> MKFKLNLITLALLANTGLAVAADGGGSDGNNGNDGSDGGEPAGSIQTLNLDITKVSYENGAPMVTVFATNEADMPVIGLANLEIKKALQLIPEGATGPGNSANWQGLGSSKSYVDNKNGSYTFKFDAFDSNKVFNAQLTQRFNVVSAAGKLADGTTVPVAEMVEDFDGQGNAPQYT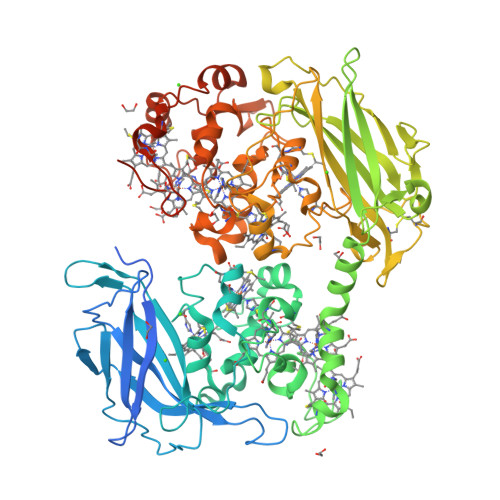KNIVSHEVCASCHVEGEKIYHQATEVETCISCHTQEFADGRGKPHVAFSHLIHNVHNANKAWGKDNKIPTVAQNIVQDNCQVCHVESDMLTEAKNWSRIPTMEVCSSCHVDIDFAAGKGHSQQLDNSNCIACHNSDWTAELHTAKTTATKNLINQYGIETTSTINTETKAATISVQVVDANGTAVDLKTILPKVQRLEIITNVGPNNATLGYSGKDSIFAIKNGALDPKATINDAGKLVYTTTKDLKLGQNGADSDTAFSFVGWSMCSSEGKFVDCADPAFDGVDVTKYTGMKADLAFATLSGKAPSTRHVDSVNMTACANCHTAEFEIHKGKQHAGFVMTEQLSHTQDANGKAIVGLDACVTCHTPDGTYSFANRGALELKLHKKHVEDAYGLIGGNCASCHSDFNLESFKKKGALNTAAAADKTGLYSTPITATCTTCHTVGSQYMVHTKETLESFGAVVDGTKDDATSAAQSETCFYCHTPTVADHTKVKMKGELKLEGKPIPNPLLGLDSTRTGHHHHHH4-[(E)-2-nitroethenyl]phenol | C8 H7 N O3 | 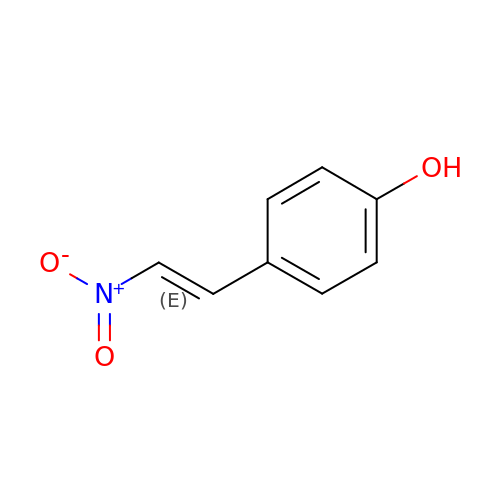CTJKRKMPTRJAIT-AATRIKPKSA-N> MIEIKDKQLTGLRFIDLFAGLGGFRLALESCGAECVYSNEWDKYAQEVYEMNFGEKPEGDITQVNEKTIPDHDILCAGFPCQAFSISGKQKGFEDSRGTLFFDIARIVREKKPKVVFMENVKNFASHDNGNTLEVVKNTMNELDYSFHAKVLNALDYGIPQKRERIYMICFRNDLNIQNFQFPKPFELNTFVKDLLLPDSEVEHLVIDRKDLVMTNQEIEQTTPKTVRLGIVGKGGQGERIYSTRGIAIGLSA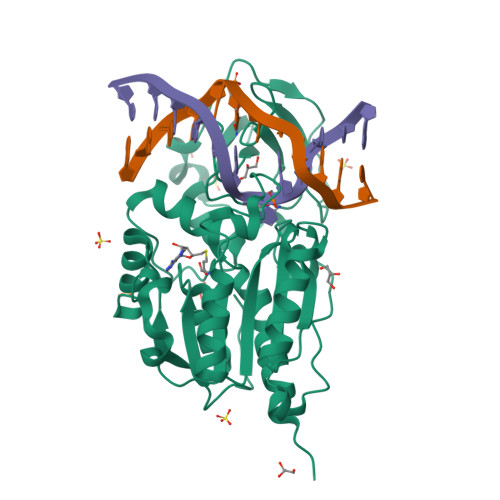YGGGIFAKTGGYLVNGKTRKLHPRECARVMGYPDSYKVHPSTSQAYKQFGNSVVINVLQYIAYNIGSSLNFKPY>GAMDPEFMDGTAAEPRPGAGSLQHAQPPPQPRKKRPEDFKFGKILGEGSFSTVVLARELATSREYAIKILEKRHIIKENKVPYVTRERDVMSRLDHPFFVKLYFCFQDDEKLYFGLSYAKNGELLKYIRKIGSFDETCTRFYTAEIVSALEYLHGKGIIHRDLKPENILLNEDMHIQITDFGTAKVLSPESKQARANSFVGTAQYVSPELLTEKSACKSSDLWALGCIIYQLVAGLPPFRAGNEYLIFQKIIKLEYDFPEKFFPKARDLVEKLLVLDATKRLGCEEMEGYGPL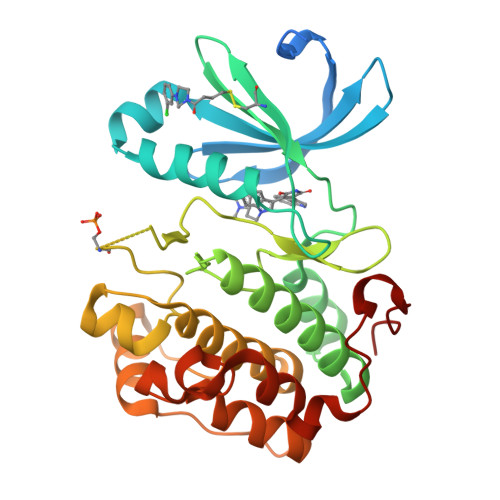KAHPFFESVTWENLHQQTPPKLT[4x]> TLLEEKVKLEEQLKETVEKYKRALADTENLRQRSQKLVEEAKLYGIQAFCKDLLEVADVLEKATQCVPKEEI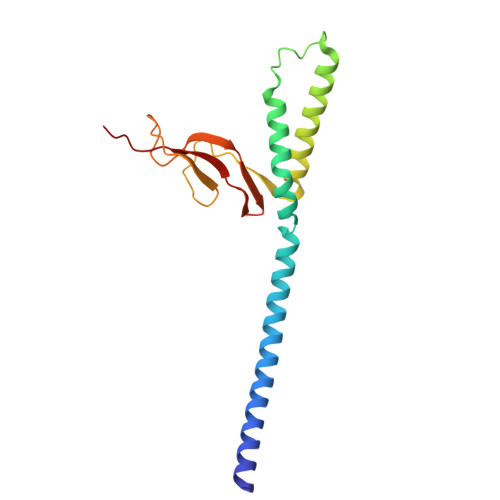KDDNPHLKNLYEGLVMTEVQIQKVFTKHGLLKLNPVGAKFDPYEHEALFHTPVEGKEPGTVALVSKVGYKLHGRTLRPALVGVVKEASA>[2x]MGSSHHHHHHSSGLVPRGSAEFHDVTEQQKIDNDRKQFVSNVSHELRTPLTSLRSYIEALSDGAWKDPEVAPGFLKVTQEETDRMIRMINELLSLSRMDSGTTRVDMELVNI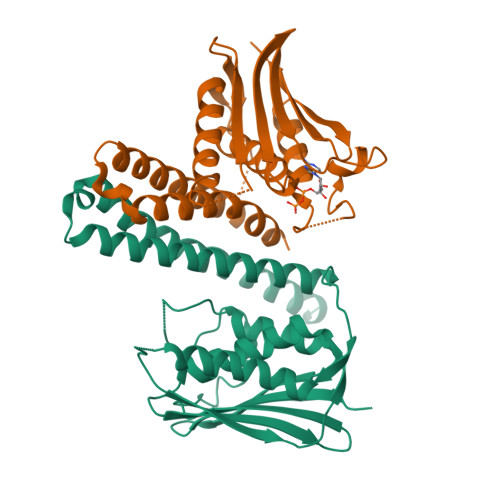NEMFNYVLDRFDMILKKDDNPAKYYTIKREFTKRDLWVEIDTDKFTQVLDNIMNNAIKYSPDGGVVTCRLLETHNQVIISISDQGLGIPRADLGHVFDRFFRVDKARSRAQGGTGLGLAISKEVVQMLGGRIWVDSVEGKGSTFYISLPYEPYEEEDLWDDDSQA>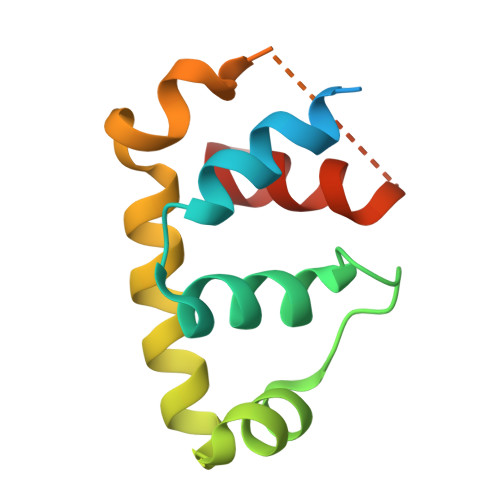 MAHHHHHHVAVDAVSFTLLQDQLQSVLDTLSEREAGVVRLRFGLTDGQPRTLDEIGQVYGVTRERIRQIESKTMSKLRHPSRSQVLRDYLDGSSGSGTPEERLLRAIFGEKA>[4x]MHHHHHHLPNITILATGGTIAGGGDSATKSNYTVGKVGVENLVNAVPQLKDIANVKGEQVVNIGSQDMNDNVWLTLAKKINTDCDKTDGFVITHGTDTMEETAYFLDLTVKCDKPVVMVGAMRPSTSMSADGPFNLYNAVVTAADKASANRGVLVVMNDTVLDGRDVTKTNTTDVATFKSVNYGPLGYIHNGKIDYQRTPARKHTSDTPFDVSKLNELPKVGIVYNYANASDLPAKALVDAGYDGIVSAGVGNGNLYKSVFDTLATAAKTGTAVVRSSRVPTGATTQDAEVDDAKYGFVASGTLNPQKARVLLQLALTQTKDPQQIQQIFNQY

The bacterial enzyme is capable of deaminating l-asparagine and, with reduced efficiency, l-glutamine, to their corresponding acidic forms releasing ammonia. The functional protein is a homotetramer and each monomer (A, B, C and D) consists of two α/β domains connected by a ca. 21 amino acid-long random-coil. The molecule includes 4 active sites, buried at the intimate dimer interface and mainly built by residues located in each protomer N-domain, as the companion C-domain of the intimate dimer contributes only one residue to the catalytic centre of the enzyme (E283′). Each active site consists of two parts: a rigid one, mainly involved in substrate binding, and a flexible one, carrying two of the six residues involved in catalysis.

Here, we report for the first time the structure of E. coli type II asparaginase in its ligand-free, open conformation (APO-EcAII) at 1.6 Å resolution with clear electron density for at least one protomer active site flexible loop, comprising key residues involved in the enzyme catalysis. The asymmetric unit (ASU) comprised 4 monomers named A, B, C, and D; chains A and B and chains C and D are associated into separated intimate dimers, each representing the functional unit of l-asparaginases. The electron density (e.d.) of residues 16–30 in chain B and of residues 16–31 in chain D was unavailable, which was consistent with most of the available structures for l-asparaginase present in the PDB. However, a clear trace of e.d. was visible for the whole loop in chain C, though with a slightly lower quality for residues G16 and G17, and for most of it in chain A (missing residues: 25–29). Compared to the closed form, the active site flexible loop has been captured in different, open orientations in two chains of the new crystal structure. In chain C, it is partially bent towards the α1 helix and its residues S23 and G28 form contacts with residues A38 and N34, respectively. In chain A, the loop is even more open, and residue T21 forms a 74.5° angle with the position of the same residue of the l-Asp-bound monomer. Apart from the active site flexible loop, all the other structural elements and the catalytically relevant residues of the APO-EcAII are superposable to the corresponding elements in the EcAII-ASP structure. The oxyanion hole described for all the l-asparaginase structures solved in complex with both L-Asp and l-Glu products, which is partially built by residues contributed by the loop in its closed position, is not evident in the new APO-EcAII structure here described. Analysis of solvent in the APO-EcAII active site pocket reveals the presence of five highly coordinated water molecules (for reference: 408, 412, 446, 529, 592 in 6YZI chain C) that interact with residues involved in l-Asp binding and are present in all 4 protomers of the ASU.> IEVWDYEQLREE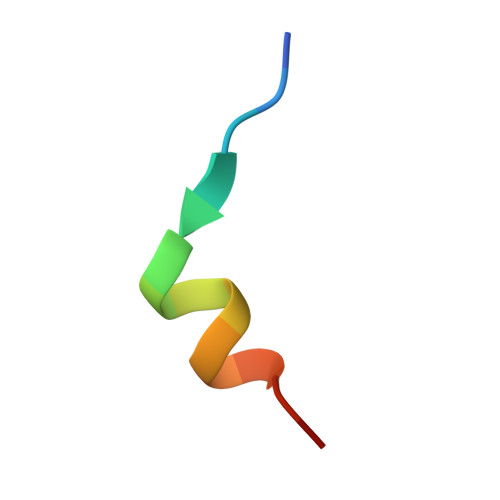YGF>[4x]MKIGVFDSGVGGFSVLKSLLKARLFDEIIYYGDSARVPYGTKDPTTIKQFGLEALDFFKPHEIELLIVACNTASALALEEMQKYSKIPIVGVIEPSILAIKRQVEDKNAPILVLGTKATIQSNAYDNALKQQGYLNISHLATSLFVPLI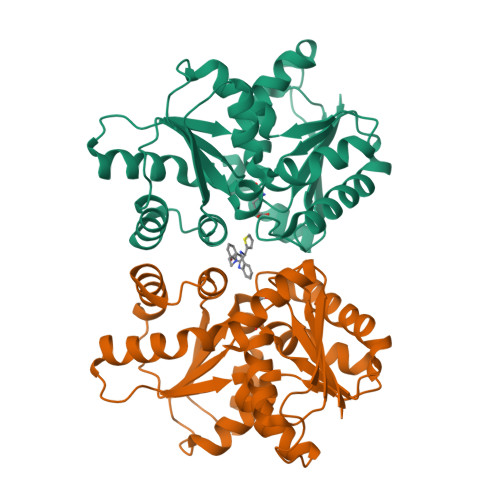EESILEGELLETCMHYYFTPLEILPEVIILGCTHFPLIAQKIEGYFMGHFALPTPPLLIHSGDAIVEYLQQKYALKNNACTFPKVEFHASGDVIWLERQAKEWLKL>GSVAGRIVIDDVQPVVSNGRYPAKAVVGEVVPVAATVWREGHDAVAATLVVRYHGTTYPDLADPPPGVPGADRTAVPIGDVMTPAAPVKPQRLPMSPGHTPDVFHGHFTPDRVGLWTYRVDGWGDPIASWRHNVTAKLDAGQGESELNNDLLVGARLLERAATGVPRELREALLEAAAALRAPGDPFTRAGAALSAEVSDLLAEYPLREFVTRGEQYGVWVDRPEARFSSWYEMFPRSTGGWDAEGRPVHGTFATAAEALPRIARMGFDVVYLPPIHPIGKVHRKGRNNSVTAAPGDVGSPWAIGSDEGGHDAVHPQLGTIEDFDEFVASARDLGLEVALDLALQCAPDHPWAREHPEWFTVLPDGSIAYAENPPKKYQDIYPLNFDNDPAGIYQEVLRVVRFWISHGVNIFRVDNPHTKPPNFWAWLIGQIKNENPDVLFLSEAFTRPARLYGLAKLGFTQSYTYFTWRTSKWELTEFGQEIAAKADIARPNLFVNTPDILHESLQHGGPGMFAIRAVLAATMGPAWGVYSGYELFENQPVRPGSEEYLNSEKYELRPRDFESALARGESLEPFLTRLNEIRRLHPALRELRTIRFHHVDNDALLAYSKFDPGTGDTVLVVVTLNPFGAEEATLWLDMPELGMEPYDRFWVRDEITGEEYQWGQANYVRLDPAKAVAHVLNMPLIPADKR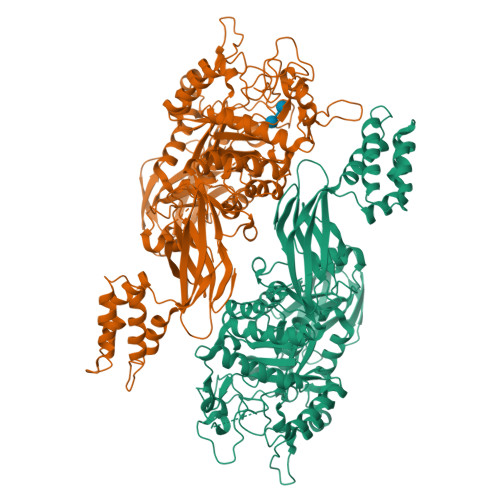LQLLRRE[2x]> GGGSGVSLEQALLILSVAALLGTTVEEAVKRALWLKTKLGVSLEQAAFILSVAAYLGTTVEEAVKRALKLKTKLGVSLEQALLILFAAAALGTTVEEAVKRALKLKTKLGVSLEQALLILWTAAELGTTVEEAVKRALKLKTKLGVSLEQAQAILVVAAELGTTVEEAVYRALKLKTKLGVSLEQAL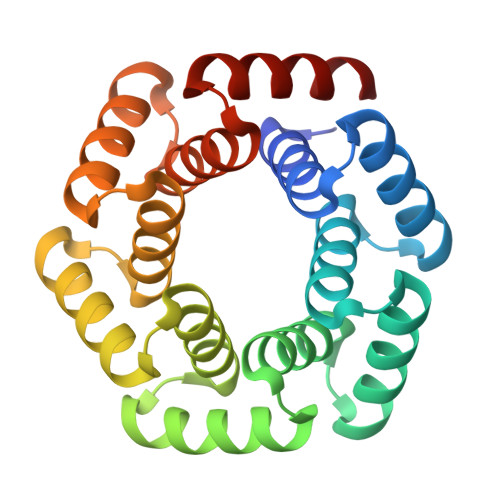LILEVAAKLGTTVEEAVKRALKLKTKLG>[2x]GESLVCKNALQDLSFLEHLLQVKYAPKTWKEQYLGWDLVQSSVSAQQKLRTQENPSTSFCQQVLADFIGGLNDFHAGVTFFAIESAYLPYTVQKSSDGRFYFVDIMTFSSE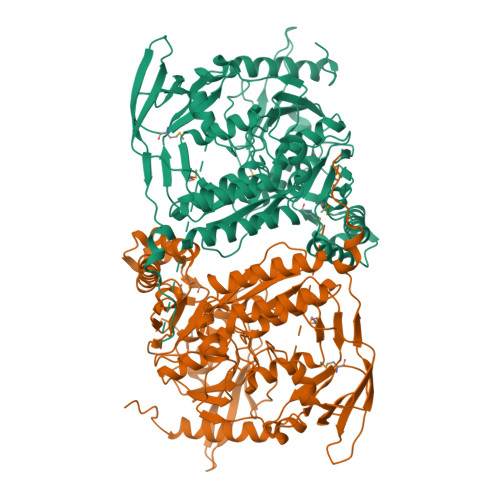IRVGDELLEVDGAPVQDVLATLYGSNHKGTAAEESAALRTLFSRMASLGHKVPSGRTTLKIRRPFGTTREVRVKWRYVPEGVGDLATIAPSIRAPQLQKSMRSFFPKKDDAFHRSSSLFYSPMVPHFWAELRNHYATSGLKSGYNIGSTDGFLPVIGPVIWESEGLFRAYISSVTDGDGKSHKVGFLRIPTYSWQDMEDFDPSGPPPWEEFAKIIQVFSSNTEALIIDQTNNPGGSVLYLYALLSMLTDRPLELPKHRMILTQDEVVDALDWLTLLENVDTNVESRLALGDNMEGYTVDLQVAEYLKSFGRQVLNCWSKGDIELSTPIPLFGFEKIHPHPRVQYSKPICVLINEQDFSCADFFPVVLKDNDRALIVGTRTAGAGGFVFNVQFPNRTGIKTCSLTGSLAVREHGAFIENIGVEPHIDLPFTANDIRYKGYSEYLDKVKKLVCQLINNDGTIILAEDGSF>SMGKLSEHLRYCDSILREMLSKKHAA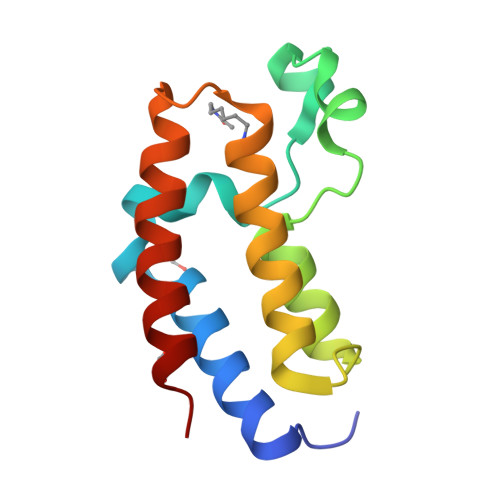YAWPFYKPVDAEALELHDYHDIIKHPMDLSTVKRKMDGREYPDAQGFAADVRLMFSNCYKYNPPDHEVVAMARKLQDVFEMRFAKMP[4x]> MHHHHHHMLEAKFEEASLFKRIIDGFKDCVQLVNFQCKEDGIIAQAVAASRVLLVSLEIGVEAFQEYRC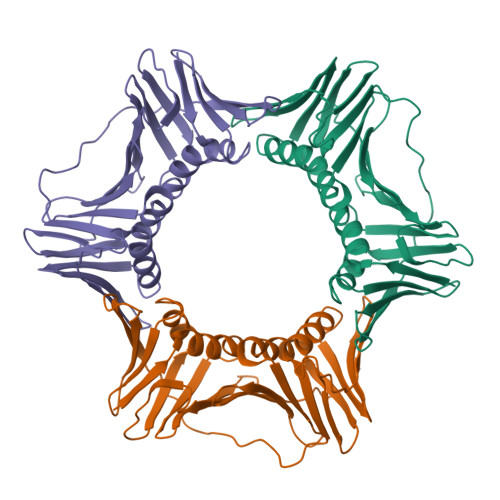DHPVTLGMDLTSLSKILRCGNNTDTLTLIADNTPDSIILLFEDTKKDRIAEYSLKLMDIDADFLKIEELQYDSTLSLPSSEFSKIVRDLSQLSDSINIMITKETIKFVADGDIGSGSVIIKPFVDMEHPETSIKLEMDQPVDLTFGAKYLLDIIKGSSLSDRVGIRLSSEAPALFQFDLKSGFLQFFLAPKFNDEE>EAVVISGRKLAQQIKQEVRQEVEEWVASGNKRPHLSVILVGENPASHSYVLNKTRAAAVVGINSETIMKPASISEEELLNLINKLNNDDNVDGLLVQLPLPEHIDERRICNAVSPDKDVDGFHVINVGRMCLDQYSML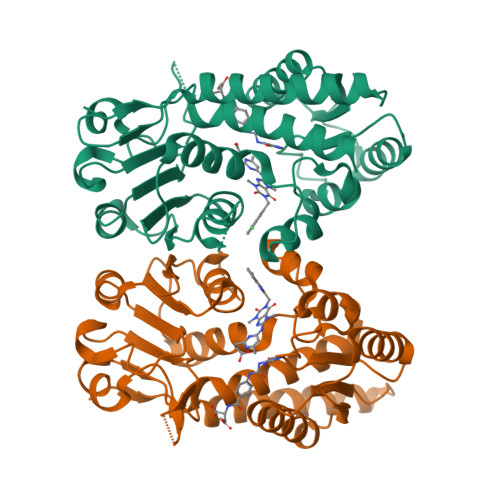PATPWGVWEIIKRTGIPTLGKNVVVAGRSKNVGMPIAMLLHTDGAHERPGGDATVTISHRYTPKEQLKKHTILADIVISAAGIPNLITADMIKEGAAVIDVGINRVHDPVTAKPKLVGDVDFEGVRQKAGYITPVPGGVGPMTVAMLMKNTIIAAKKVLRLEEREVLKSKELGVATN[2x]>MRVVLIVDIVRQEEKLIAKALEENKVQYDIINVAQEPLPFNKALGRYDVAIIRPVSMYRALYSS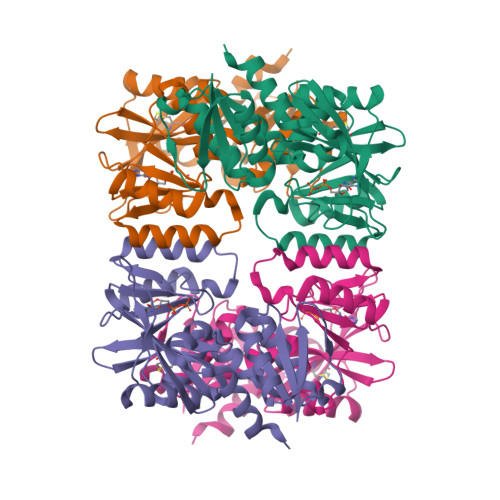AVLEAAGVHTINSSDVINVCGDKILTYSKLYREGIPIPDSIIALSAEAALKAYEQRGFPLIDKPPIGSWGRLVSLIRDVFEGKTIIEHRELMGNSALKAHIVQEYIQYKGRDIRCIAIGEELLGCYARNIPPNEWRANVALGGTPSNIEVDEKLKETVVKAVSIVHGEFVSIDILEHPNKGYVVNELNDVPEFKGFMVATNINVAQKLVEYIKENYSK[4x]> MGLFDRLGRVVRANLNDLVSKAEDPEKVLEQAVIDMQEDLVQLRQAVARTIAEEKRTEQRLNQDTQEAKKWEDRAKLALTNGEENLAREALARKKSLTDTAAAYQTQLAQQRTMSENLRRNLAALEAKISEAKTKKNMLQARAKAAKANAELQQTLGGLGTSSATSAFERMENKVLDMEATSQAAGELAGFGIENQFAQLEASSGVEDELAALKASMAGGALPGTSAATPQLEAAPVDSSVPANNASQDDAVIDQELDDLRRRLNNLAALEVLFQGP

A prominent member of the PspA family is the vesicle-inducing protein in plastids 1 (Vipp1), also known as IM30 (inner membrane-associated protein of 30 kDa). Vesicle-inducing protein in plastids 1 (Vipp1) is critical for thylakoid membrane biogenesis and maintenance. Vipp1 appears to have two functions: in membrane maintenance (that is, during heat or light stress) and in thylakoid membrane (TM) biogenesis and/or remodeling. Vipp1 binds to negatively charged membranes and membrane binding depends on stored curvature elastic stress.

Using single-particle-based helical reconstruction, we resolved the structures of type I tubes at 5.1-Å resolution and two structures of type II tubes at 7.0-Å and 7.1-Å resolution. The type I and II tubes differ in their diameter and the arrangement of the monomers relative to the tube axis, as well as the diameter and thickness of the engulfed lipid bilayer tube. In contrast to the Vipp1 rings, the monomer orientation of the α1−α3 hairpin with respect to the tube axis is the same over the whole length of the tubes. Nevertheless, the monomer orientation among the tubes differs; in type I tubes, the α1−α3 hairpins are oriented parallel to the tube axis, while, in type II tubes, the hairpins are tilted approximately 45° relative to the tube axis. Remarkably, from rings over type II tubes to type I tubes, the α1−α3 hairpins accommodate a wide range of orientations along the tubulated membrane axis from perpendicular to parallel (from 90° to 0°) while essentially maintaining the same intermolecular contacts to stabilize the assembly. The here-determined structures of Vipp1 polymers in the presence of membranes indicated that helix α0 is immersed in the outer lipid leaflet of the bilayer. However, in contrast to SynPspA helix α0 that protrudes toward the bilayer, Vipp1 α0 lies flat in the membrane plane and appears to be partially submerged into the outer bilayer leaflet. The bilayer thickness in all three Vipp1 tubes remained nearly identical at 35 Å, although the inner leaflet radius changed with the tube diameter. Nevertheless, the same or similar intermolecular interactions of α0 with another α0 and α1 + α4, as observed previously in Vipp1 rings, are present in type I and II tubes.> MKKYVCTVCGYEYDPAEGDPDNGV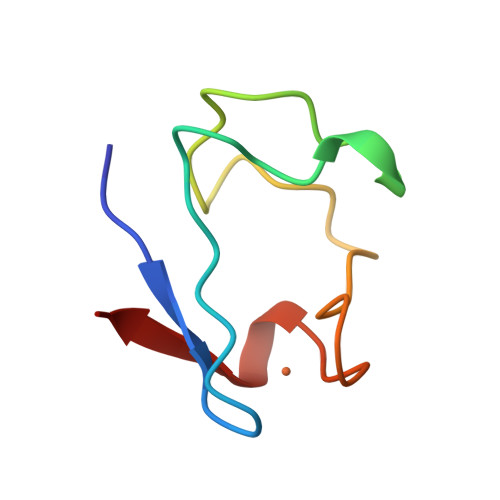KPGTAFEDVPADWVCPICGAPKSEFEPA>[2x]AMNYFVGNSLGVNLTGIEKAIINRLNLFKEMGRPAQCVFLSWNRYLYRNAQNYITSSDYINMYDFFQEATYLERNEPFDWLSYWTDECHYTLKHVENSHDFRIYDQERFLMY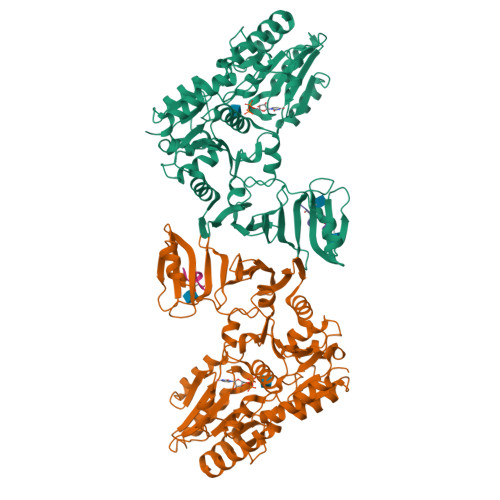AHFQDPKYRILDYVNHFDSQRRKVKRDFYDVRGFLSCSRILVDKQQTLCEFFYNPEGDTKLEKYFSYKDGKPEVQKIIVYYANKQYFFNNETELGAFFIKQLYQHGDLFFSDRNVYTAPIFNLTPESIPVVAVLHSTHIKNIDALDSSPFKNVYKAMFENLSRYRAIIVSTEQQKLDVEKRINHTIPVVNIPVGYSETIDTPVQTLDQRSVKLISVARYSPEKQLHQQIELIKRLVSYVPKIELHMYGFGSESKKLNELIQKYGLENHVYLRGFLSNLDQEYSDAYLSLITSNMEGFSLALLESLAHGVPVISYDIKYGPNELITSDFNGYLITKNDEDALFDKVKYVIDHPEVQQRLSKGSLAKAQQYSKASLIKQWDQFVRLILEHHHHHH;>SDSDSDSD[2x]N-{4-chloro-5-[1-ethyl-7-(methylamino)-2-oxo-1,2-dihydro-1,6-naphthyridin-3-yl]-2-fluorophenyl}-N'-phenylurea 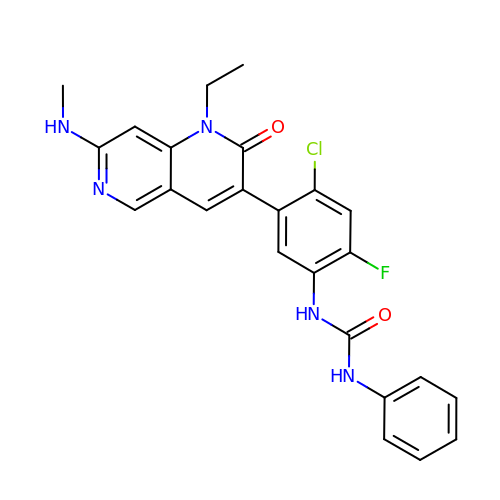| C24 H21 Cl F N5 O2 | VWSRPILDGFSBIY-UHFFFAOYSA-N>[3x]SRCTHLENRDFVTGTQGTTRVTLVLELGGCVTITAEGKPSMDVWLDAIYQENPAQTREYCLHAKLSDTKVAARCPTMGPATLAEEHQGGTVCKRDQSDRGWGNHCGLFGKGSIVACVKAACEAKKKATGHVYDANKIVYTVKVEPHTGDYVAANETHSGRKTASFTVSSEKTILTMGEYGDVSLLCRVASGVDLAQTVILELDKTVEHLPTAWQVHRDWFNDLALPWKHEGARNWNNAERLVEFGAPHAVKMDVYNLGDQTGVLLKALAGVPVAHIEGTKYHLKSGHVTCEVGLEKLKMKGLTYTMCDKTKFTWKRAPTDSGHDTVVMEVTFSGTKPCRIPVRAVAHGSPDVNVAMLITPNPTIENNGGGFIEMQLPPGDNIIYVGELSYQWFQKGSSIGRVFQKTKKGIERLTV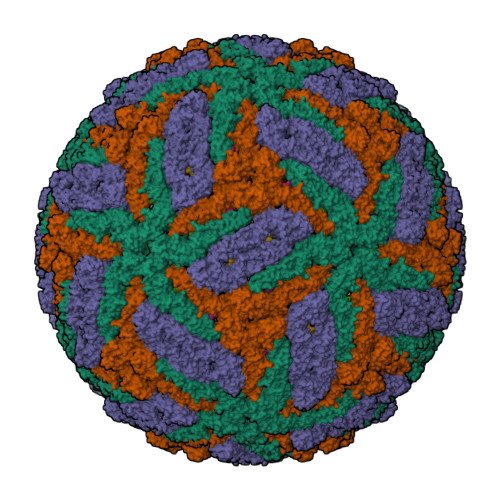IGEHAWDFGSAGGFLSSIGKALHTVLGGAFNSIFGGVGFLPKLLLGVALAWLGLNMRNPTMSMSFLLAGVLVLAMTLGVGA;>[3x]SVLIPSHAQGELTGRGHKWLEGDSLRTHLTRVEGWVWKNRLLALAMVTVVWLTLESVVTRVAVLVVLLCLAPVYA> DHINLKVAGQDGSVVQ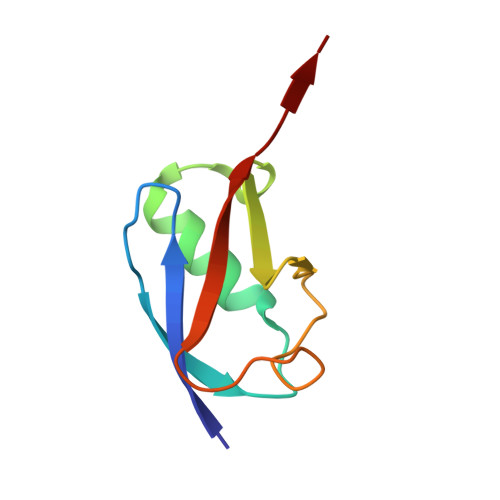FKIKRHTPLSKLMKAYCERQGLSMRQIRFRFDGQPINETDTPAQLEMEDEDTIDVFQQQTGG> FIFLALLGAAVAFPVDDDDKIVGGYTCGANTVPYQVSLNSGYHFCGGSLINSQWVVSAAHCYKSGIQVRLGEDNINVVEGNEQFISASKSIVHPSYNSNTLNNDIMLIKLKSAASLNSRVASISLPTSC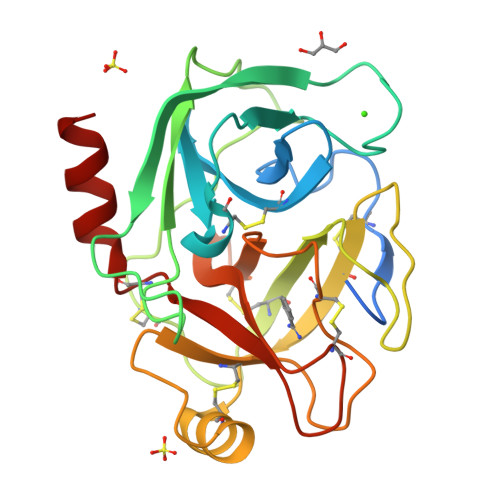ASAGTQCLISGWGNTKSSGTSYPDVLKCLKAPILSDSSCKSAYPGQITSNMFCAGYLEGGKDSCQGDSGGPVVCSGKLQGIVSWGSGCAQKNKPGVYTKVCNYVSWIKQTIASN2-(2-fluorophenyl)-N-[(5-methylthiophen-2-yl)methyl]ethanamine | 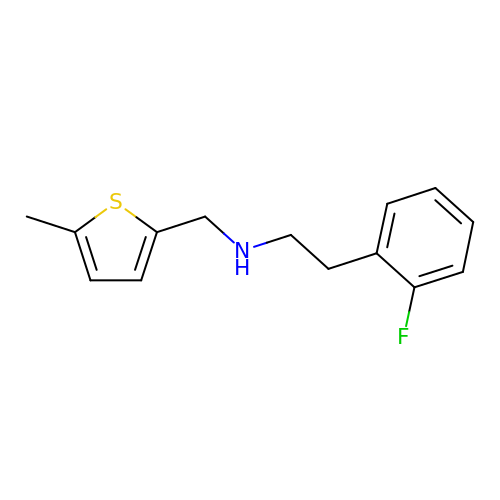C14 H16 F N S | NZNHJQFNTSWMCR-UHFFFAOYSA-N> MNSLSSKKANSLVFKSIRNFTLQWGSLAERPMVDRVMSTSTWPVPYYQRLFKAYPIREKKDKMSLLLSDIDIDDTNWYQAKDFLRGSFRGRQIVDYVENNIASNTYILIQQDVANMAKAYVHDICGYIDV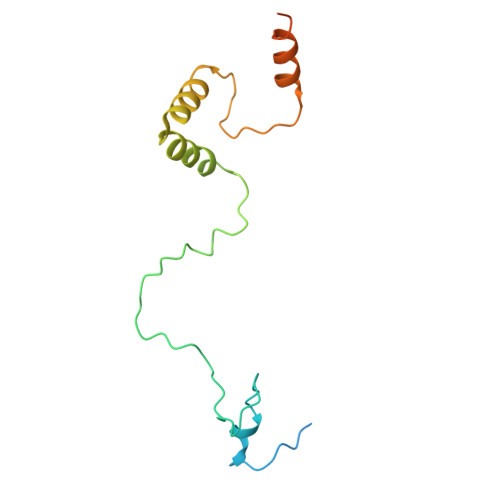ANKENVRILSKGDLI>MEIYLVTGNMNKKEEFLKMMDEELNVEFVNINLEEIQAQDIVEINEHKVKTAYNILKKQDNNKNKKRYVITDDTGLFISKLNNFPGPYIKWMQKALGSKGIADVVSRLDDNTCHAICTYSVYDGKDVHSFKGITNGKIVEPRGNNKFGWDNIFQPESLSKTFGEMTFDEKQNLSPRFKAFVQLKEFLMNEHKKYN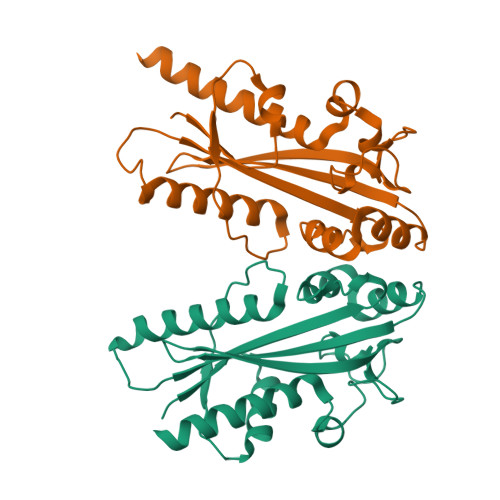NEF[2x]>[4x]MGSSHHHHHHSSGRENLYFQGMELLKHLSQRQYIDGEWVESANKNTRDIINPYNQEVIFTVSEGTKEDAERAILAARRAFESGEWSQETAETRGKKVRAIADKIKEHREALARLETLDTGKTLEESYADMDDIHNVFMYFAGLADKDGGEMIDSPIPDTESKIVKEPVGVVTQITPWNYPLLQASWKIAPAL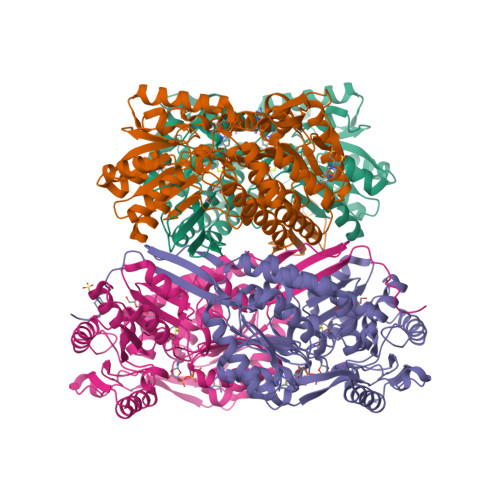ATGCSLVMKPSEITPLTTIRVFELMEEVGFPKGTINLILGAGSEVGDVMSGHKEVDLVSFTGGIETGKHIMKNAANNVTNIALELGGKNPNIIFDDADFELAVDQALNGGYFHAGQVCSAGSRILVQNSIKDKFEQALIDRVKKIKLGNGFDADTEMGPVISTEHRNKIESYMDVAKAEGATIAVGGKRPDRDDLKDGLFFEPTVITNCDTSMRIVQEEVFGPVVTVEGFETEQEAIQLANDSIYGLAGAVFSKDIGKAQRVANKLKLGTVWINDFHMYFAQAPWGGYKQSGIGRELGKEGLEEYLVSKHILTNTNPQLVNWFSK>MSAIENFDAHTPMMQQYLRLKAQHPEILLFYRMGDFYELFYDDAKRASQLLDISLTKRGASAGEPIPMAGIPYHAVENYLAKLVNQGESVAICEQIGDPATSKGPVERKVVRIVTPGTISDEALLQERQDNLLAAIWQDSKGFGYATLDISSGRFRLSEPADRETMAAELQRTNPAELLYAEDFAEMSLIEGRRGLRRRPLWEFEIDTARQQLNLQFGTRDLVGFGVENAPRGLCAAGCLLQYAKDTQRTTLPHIRSITMEREQDSIIMDAATRRNLEITQNLAGGAENTLASVLDCTVTPMGSRMLKRWLHMPVRDTRVLLERQQTIGALQDFTAGLQPVLRQVGDLERILARLALRTARPRDLARMRHAFQQLPELRAQLETVDSAPVQALREKMGEFAELRDLLERAIIDTPPVLVRDGGVIASGYNEELDEWRALADGATDYLERLEVRERERTGLDTLKVGFNAVHGYYIQISRGQSHLAPINYMRRQTLKNAERYIIPELKEYEDKVLTSKGKALALEKQLYEELFDLLLPHLEALQQSASALAELDVLVNLAERAYTLNYTCPTF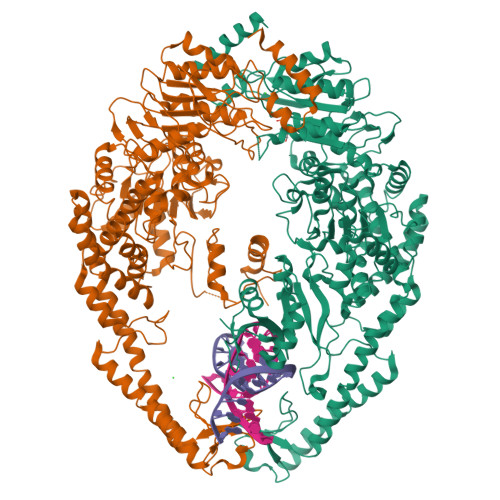IDKPGIRITEGRHPVVEQVLNEPFIANPLNLSPQRRMLIITGPNMGGKSTYMRQTALIALMAYIGSYVPAQKVEIGPIDRIFTRVGAADDLASGRSTFMVEMTETANILHNATEYSLVLMDEIGRGTSTYDGLSLAWACAENLANKIKALTLFATHYFELTQLPEKMEGVANVHLDALEHGDTIAFMHSVQDGAASKSYGLAVAALAGVPKEVIKRARQKLRELESIS[2x]>MQQASTPTIGMIVPPAAGLVPADGARLYPDLPFIASGLGLGSVTPEGYDAVIESVVDHARRLQKQGAAVVSLMGTSLSFYRGAAFNAALTVAMREATGLPCTTMSTAVLNGLRALGVRRVALATAYIDDVNERLAAFLAEESLVPTGCRSLGITGVEAMARVDTATLVDLCVRAFEAAPDSDGILLSCGG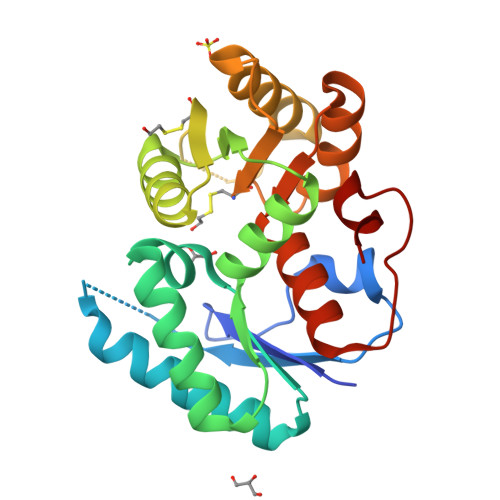LLTLDAIPEVERRLGVPVVSSSPAGFWDAVRLAGGGAKARPGYGRLFDES[4x]> GAGESITAVGSTALQPLVEAAGEQYTGEHLGTFINVQGGGTGTGLSQIQEGA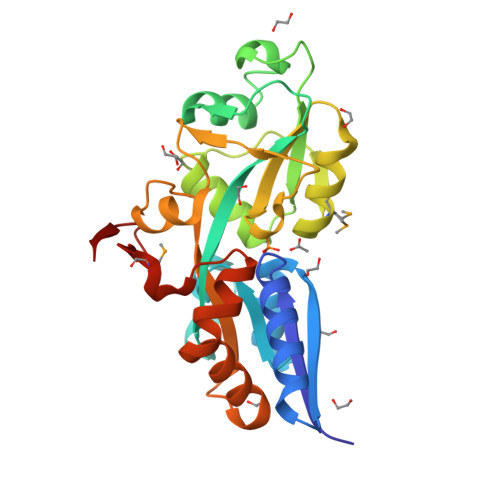VQIGNSDLFAGEQKGINARQLVDHRVAVVGITPIVNKKVGVKNLSTNQLIKIFTGQITNWKEVGGADQSIVLINRAQGSGTRATFEQFGLANHRSKTAQEQDSSGMVRSIVATTPGAISYVAFSYVNKTVQALSLNHVAPTEVNVTTNDWRIWSYEHLYTKGHPTGLTKAFITYVQSPAIQNTLVRQLGYLSPDQMLVERDANGHITKTGGA> MLPLYLLTNAKGQQMQIELKNGEIIQGILTNVDNWMNLTLSNVTEYSEESAINSEDNAES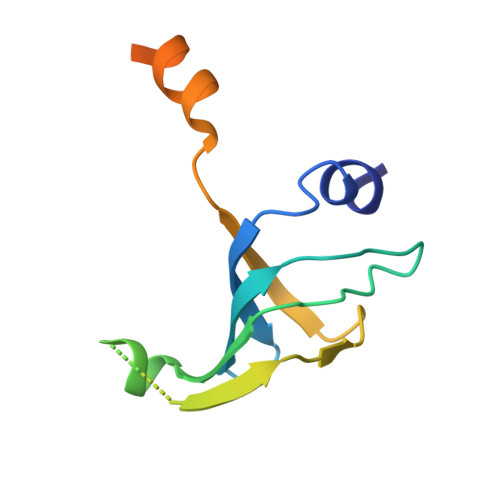SKAVKLNEIYIRGTFIKFIKLQDNIIDKVKQQINSNNNSNSNGPGHKRYYNNRD(2R)-2-amino-3-(2,4-dichlorophenyl)-1-(1,3-dihydro-2H-isoindol-2-yl)propan-1-one | C17 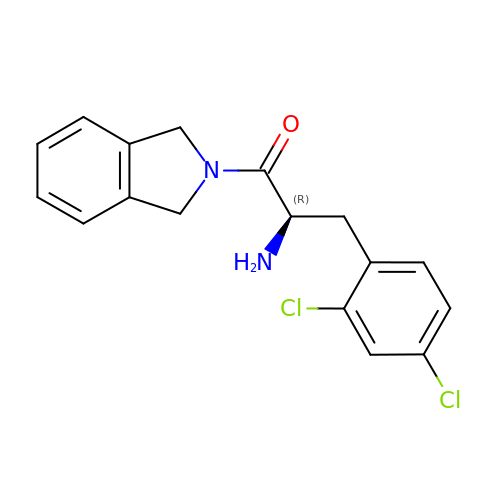H16 Cl2 N2 O | JFWNERIMAUEHNN-MRXNPFEDSA-N> MSLYTILV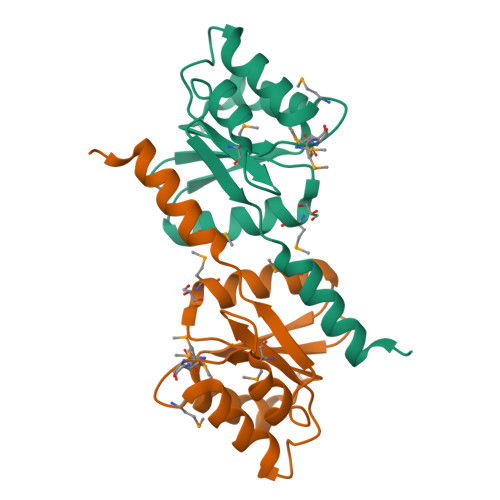VDDSPMIVDVFVTMLERGGYRPITAFSGEECLEALNATPPDLVLLDIMMEPMDGWETLERIKTDPATRDIPVLMLTAKPLTPEEANEYGSYIEDYILKPTTHHQLYEAIEHVLARRHSIAADEGHHHHHH(2S)-oxetane-2-carboxylic 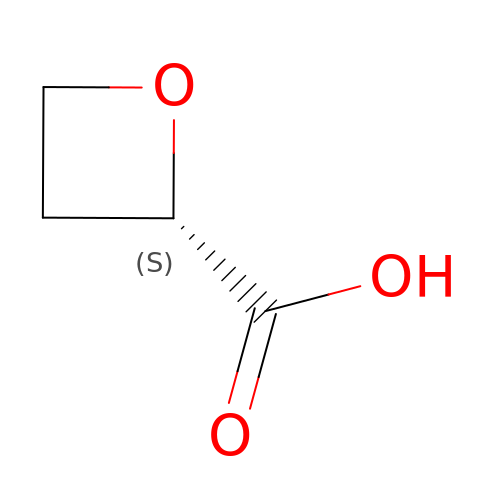acid | C4 H6 O3 | ZKCXAZCRQJSFTQ-VKHMYHEASA-N1-[4-(4-chlorophenyl)piperazin-1-yl]ethan-1-one 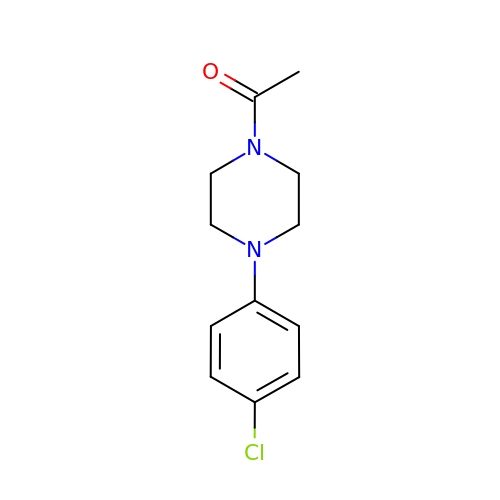| C12 H15 Cl N2 O | UVYFWYMZWQBGAQ-UHFFFAOYSA-N> EDRPIKFSTEGATSQSYKQFIEALRERLRGGLIHDIPVLPDPTTLQERNRYITVELSNSDTESIEVGIDVTNAYVVAYRAGTQSYFLRDAPSSASDYLFTGTDQHSLPFYGTYGDLERWAHQSRQQIPLGLQALTHGISFFRSGGNDNEEKARTLIVIIQMVAEAARFRYISNRVRVSIQTGTAFQPDAAMISLENNWDNLSRGVQESVQDTFPNQVTLTNIRNEPVIVDSLSHPTVAVLALMLFVCNPPN;> IVEKSKICSSRYEPTVRIGGRDGMCVDVYDNGYHNGNRIIMWKCKDRLEENQLWTLKSDKTIRSNGKCLTTYGYAPGSYVMIYDCTSAVAEATYWEIWDNGTIINPKSALVLSAESSSMGGTLTVQTNEYLMRQGWRTGNNTSPFVTSISGYSDLCMQAQGSNVWMADCDSNKKEQQWALYTDGSIRSVQNTNNCLTSKDHKQGSTILLMGCSNGWASQRWVFKNDGSIYSLYDDMVMDVKGSDPSL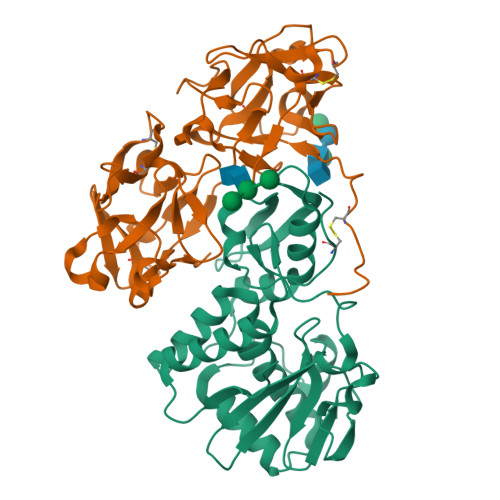KQIILWPYTGKPNQIWLTLF>SLSTGCYMVKQGPTSVAYVEVNNNSMLNVGKYTLADGGGNAFDVAVIFAANINYDTGTKTAYLHFNENVQRVLDNAVTQIRPLQQQGIKVLLSVLGNHQGAGFANFPSQQAASAFAKQLSDAVAKYGLDGVDFDDEYAEYGNNGTAQPNDSSFVHLVTALRANMPDKIISLYNIGPAASRLSYGGVDVSDKFDYAW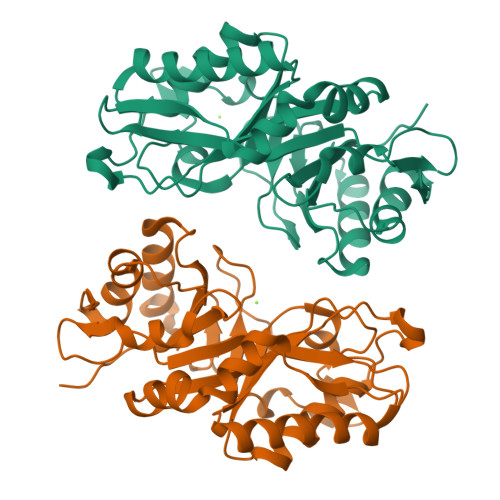NPYYGTWQVPGIALPKAQLSPAAVEIGRTSRSTVADLARRTVDEGYGVYLTYNLDGGDRTADVSAFTRELYGSEAVRTPHHHHHH[4x]> MSSFYTVVGVFIVVSAMSVLFWIMAPKNNQAVWRSTVILTLAMMFL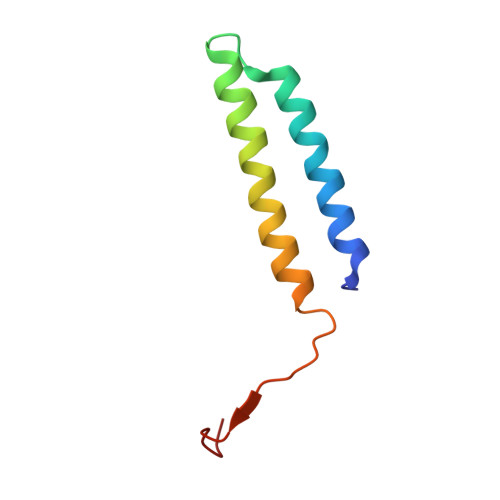MWAITFLCQLHPLVAPRRSDLRPEF Arabidopsis MORPHEUS' MOLECULE1 (MOM1) is an exceptional TGS regulator that acts largely independently of changes in the levels of DNA methylation and H3K9me2. MOM1 is a large nuclear protein of 2001 amino acids containing an incomplete and highly degenerate helicase domain related to a similar domain found in CHD3 chromatin-remodeling factors. Surprisingly, only the predicted nuclear localization signal (NLS) and a short fragment of MOM1 of less than 200 amino acids (1663 to 1859) containing a conserved plant-specific motif of 82 amino acids (1734 to 1815), named Conserved MOM1 Motif 2 (CMM2), is required for TGS activity. We solved the structure of this domain and found that it forms a dimer with each monomer consisting of unusual consecutive 11 amino-acid hendecad repeats folding into an antiparallel coiled-coil.

The best diffracting crystals were obtained with a MOM1 fragment corresponding to amino acid positions 1700 to 1814 (for experimental details, see [26] and Materials and methods) and a complete dataset was collected to a maximal resolution of 3.2 Å. A poor electron density map, most likely the result of the absence of stable secondary structure, prevented us from building the first 28 as well as the last 3 amino acids of the CMM2-containing fragment. The structure reveals that the CMM2 motif folds as a long α-helix. Two such helices form an antiparallel coiled-coil structure. The asymmetric unit contains two identical coiled-coils that further interact via their N- and C-termini to form the crystal lattice. The mutual association of two CMM2 monomers occurs mainly through a large interface formed by hydrophobic residues. Additional stabilization of the coiled-coil comes from an intermolecular network of salt bridges established between glutamate and lysine residues. In contrast to the classical coiled-coil structure, CMM2 monomers are not wound around each other and, therefore, do not generate a left-handed super-coil. The CMM2 fragment forms dimeric coiled-coils with extensive hydrogen bonds or salt bridges mediating inter-chain contacts via residues at positions g and k.

>HSAGVTALVPSLLNNGTEQIAVQPVPQIPFPVFNDPFLHELEKLRRESENSKKTFEEKKSILKAELERKMAEVQAEFRRKFHEVEAEHNTRTTKIEKDKNLVIMNKLLANAFLSK[4x]> MTLEDLQLLADLFYLPYEHGPKGAQMLREFQWLRANSSVVSVNCKGKDSEKIEEWRSRAAKFEEMCGLVMGMFTRLSNCANRTILYDMYSYVWDIKSIMSMVKSFVQWLGCRSHSSAQFLIGDQEPWAFRGGLAGEFQR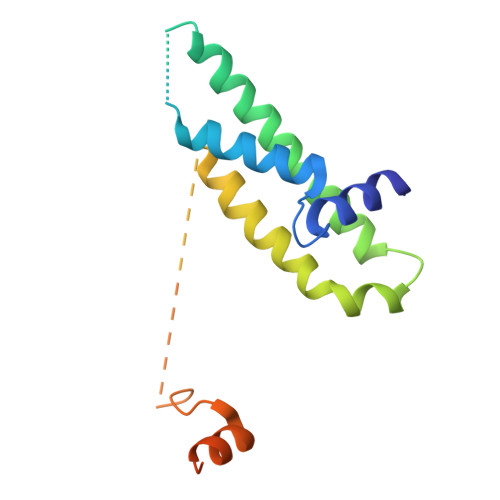LLPIDGANDLFFQPHHHHHHHH>[6x]KLPYKVADIGLAAWGRKALDIAENEMPGLMRMRERYSASKPLKGARIAGCLHMTVETAVLIETLVTLGAEVQWSSCNIFSTQDHAAAAIAKAGIPVYAWKGETDEEYLWCIEQTLYFKDGPLNMILDDGGDLTNLIHTKYPQLLPGIRGISEETTTGVHNLYKMMANGILKVPAINVNDSVTKSKFDNLYGCRESLIDGIKR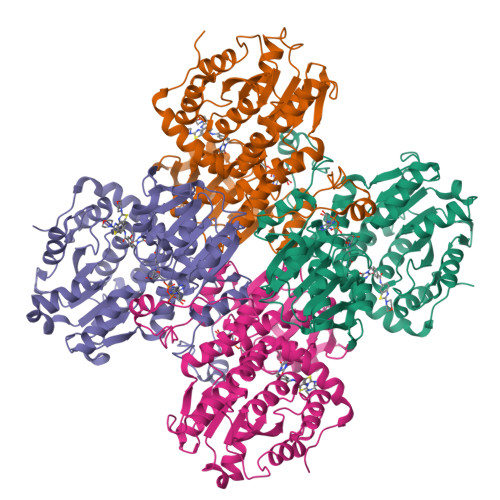ATDVMIAGKVAVVAGYGDVGKGCAQALRGFGARVIITEIDPINALQAAMEGYEVTTMDEACQEGNIFVTTTGCIDIILGRHFEQMKDDAIVCNIGHFDVEIDVKWLNENAVEKVNIKPQVDRYRLKNGRRIILLAEGRLVNLGCAMGHPSFVMSNSFTNQVMAQIELWTHPDKYPVGVHFLPKKLDEAVAEAHLGKLNVKLTKLTEKQAQYLGMSCDGPFKPDHYRY>MDVEAFYKISYGLYIVTSESNGRKCGQIANTVFQLTSKPVQIAVCLNKENDTHNAVKESGAFGVSVLELETPMEFIGRFGFRKSSEFEKFDGVEYKTGKTGVPLVTQHAVAVIEAKVVKECDVGTHTLFVGEAVDAEVLKDAEVLTYADYHLMKKG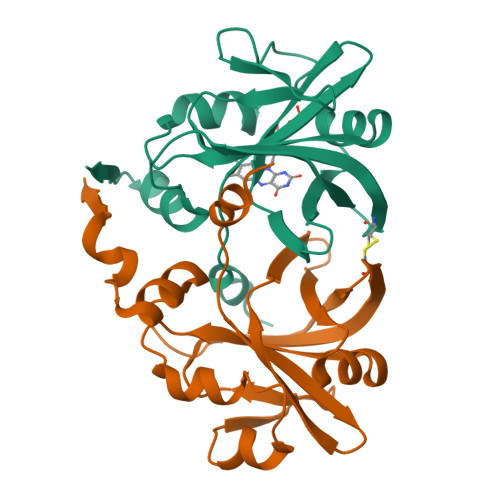KTPRTATVYFESK[2x]> GSQIPASEQETLVRPKPLLLKLLKSVGAQKDTYTMKEVLFYLGQYIM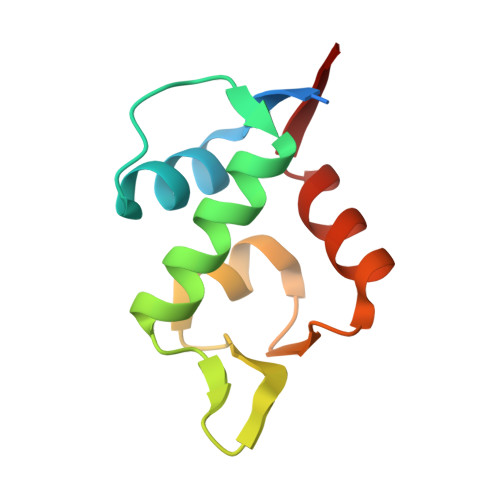TKRLYDEKQQHIVYCSNDLLGDLFGVPSFSVKEHRKIYTMIYRNLVVVN3-{[(E)-AMINO(HYDROXYIMINO)METHYL]AMINO}PROPAN-1-AMINIUM | C4 H13 N4 O | 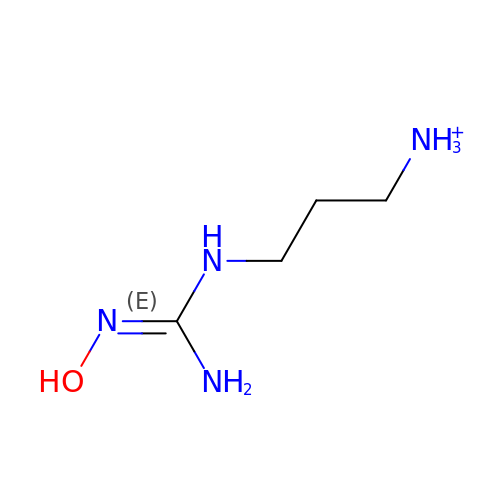HYBLXYGPQAIGPY-UHFFFAOYSA-O>MSIKIRDFGLGSDLISLTNKAGVTISFTNLGARIVDWQKDGKHLILGFDSAKEYLEKDAYPGATVGPTAGRIKDGLVKISGKDYILNQNEGPQTLHGGEESIHTKLWTYEVTDLGAEVQVKFSLVSNDGTNGYPGKIEMSVTHSFDDDNKWKIHYEAISDKDTVFNPTGHVYFNLNGDASESVENHGLRLAASRFVPLKDQTEIVRGDIVDIKNTDLDFRQEKQLSN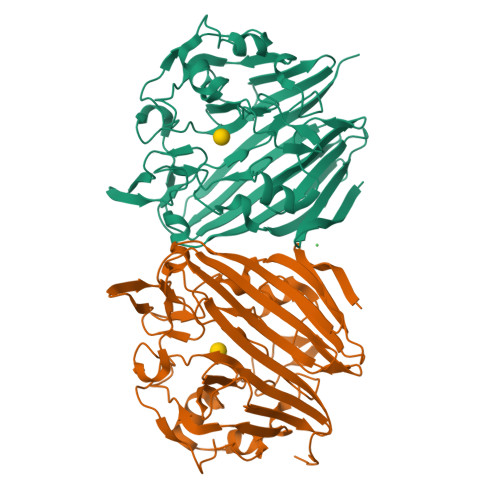AFNSNMEQVQLVKGIDHPFLLDQLGLDKEQARLTLDDTSISVFTDQPSIVIFTANFGDLGTLYHEKKQVHHGGITFACQVSPGSEQIPELGDISLKAGEKYQATTIYSLHTKLEHHHHHH[2x]>MHRTSNGSHATGGNLPDVASHYPVAYEQTLDGTVGFVIDEMTPERATASVEVTDTLRQRWGLVHGGAYCALADMLATEATVAVVHEKGMMAVGQS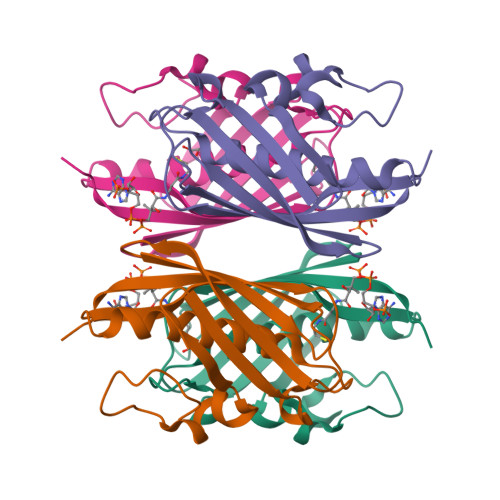NHTSFFRPVKEGHVRAEAVRIHAGSTTWFWDVSLRDDAGRLCAVSSMSIAVRPRRD[2x]> IVGGQECKDGECPWQALLINEENEGFCGGTILSEFYILTAAHCLYQAKRFKVRVGDRNTEQEEGGEAVHEVEVVIKHNRFTKETYDFDIAVLRLKTPITFRMNVAPACLPERDWAESTLMTQKTGIVSGFGRTHEKGRQSTRLKM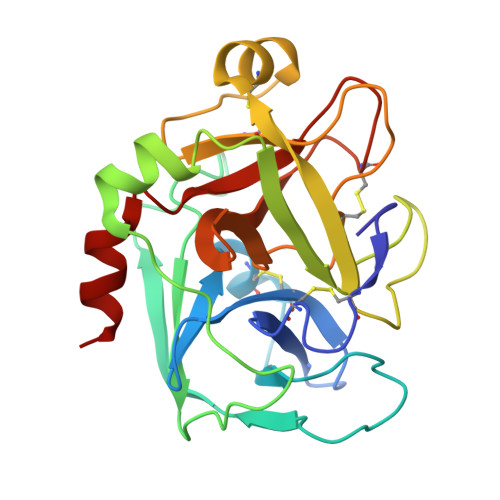LEVPYVDRNSCKLSSSFIITQNMFCAGYDTKQEDACQGDSGGPHVTRFKDTYFVTGIVSWGEGCARKGKYGIYTKVTAFLKWIDRSMK9-(2-chloranyl-7~{H}-pyrrolo[2,3-d]pyrimidin-4-yl)-4-[4-[(4,4-dimethylpiperidin-1-yl)methyl]phenyl]-1,4,9-triazaspiro[5.5]undecan-2-one | 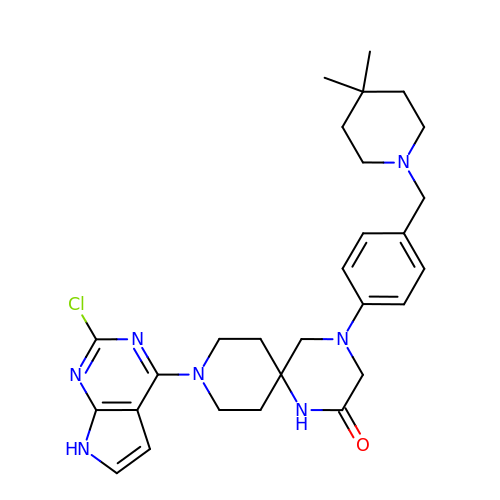C28 H36 Cl N7 O | QFCRIUPWCMVQHW-UHFFFAOYSA-N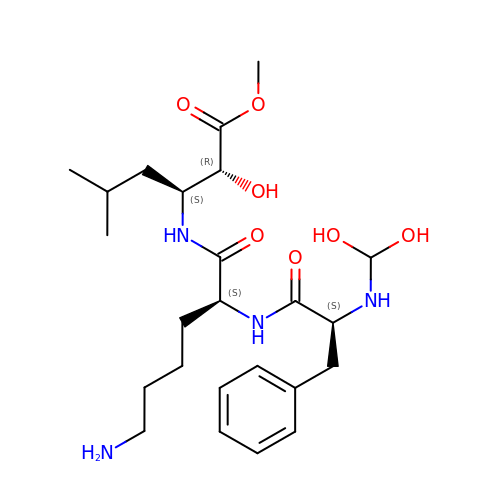N-(dihydroxymethyl)-L-phenylalanyl-N-[(2R,3S)-2-hydroxy-1-methoxy-5-methyl-1-oxohexan-3-yl]-L-lysinamide | C24 H40 N4 O7 | FKYXTMPITQBLQQ-LWYYNNOASA-N>[4x]MVYVSNKYLTMSEMKVNAQYILNYLSSNGWTKQAICGMLGNMQSESTINPGLWQNLDEGNTSLGFGLVQWTPASNYINWANSQGLPYKNMDSELKRIIWEVNNNAQWINLRDMTFKEYIKSTKTPRELAMIFLASYERPANPNQPERGDQAEYWYKNLSGGGGGGLQLAQFPMDIINISQGENGSFSHKGTLCIDFVGKTEKYPYYAPCDCTCVWRGDASAYLAWTSDKEVMC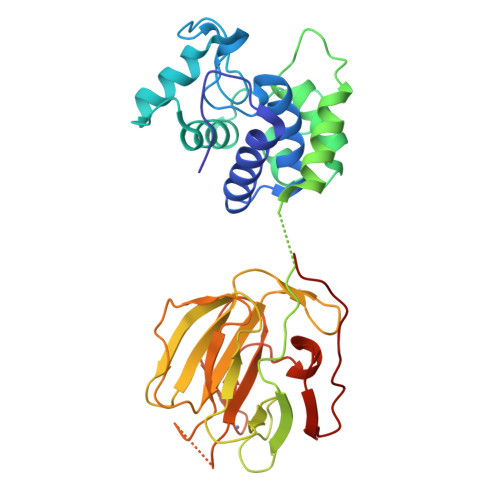ADGSVRYITWVNVHESPLPFDVGKKLKKGDLMGHTGIGGNVTGDHWHFNVIDGKEYQGWTKKPDSCLAGTELHIYDVFAVNNVEIINGNGYDWKTSDWQDG> GSMSAKDERAREILRGFKLNWMNLRDAETGKILWQGTEDLSVPGVEHEARVPKKILKCKAVSRELNFSSTEQMEKFRLEQKVYFKGQCLEEWFFEFGFVIPNSTNTWQSLIEAAPESQMMPASVLTGNVIIETKFFDDDLLVSTSRVRLFYV;> LMPDSGAVFTFGKSKFAENNPGKFWFKNDVPVHLSCGDEHSAVVTGNNKLYMFGSNNWGQLGLGSKSAISKPTCVKALKPEKVKLAACGRNHTLVSTEGGNVYATGGNNEGQLGLGDTEE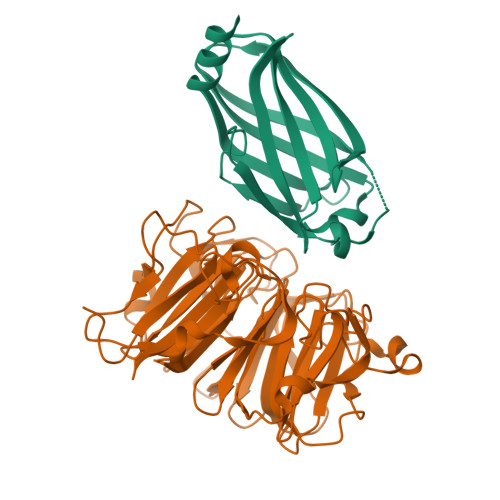RNTFHVISFFTSEHKIKQLSAGSNTSAALTEDGRLFMWGDNSEGQIGLKNVSNVCVPQQVTIGKPVSWISCGYYHSAFVTTDGELYVFGEPENGKLGLPNQLLGNHRTPQLVSEIPEKVIQVACGGEHTVVLTENAVYTFGLGQFGQLGLGTFLFETSEPKVIENIRDQTISYISCGENHTALITDIGLMYTFGDGRHGKLGLGLENFTNHFIPTLCSNFLRFIVKLVACGGCHMVVFAAPHPRRPPAYVEQKLISEEDLNSAVDHHHHHH> PNFSGNWKIIRSENFEELLKVLGVNVMLRKIAVAAASKPAVEIKQEGDT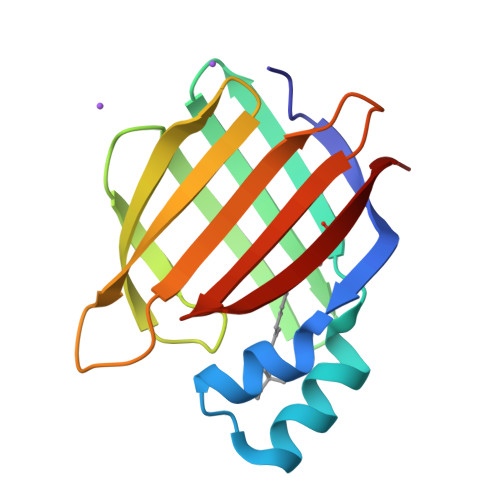FYIKTSTTVRTTEINFKVGEEFEEQTVDGRPCKSLVKWESENKMVCEQKLLKGEGPKTSWTLELTNDGELIETMTADDVVCTKVYVRE Acetobacter aceti strain 1023 and other acetic acid bacteria use succinyl-CoA:acetate CoA-transferase (AarC) in a variant citric acid cycle that is required for a robust acetic acid resistance (aar) phenotype. Strong selection for key roles in acetic acid resistance and central metabolism appear to have optimized the structural and functional properties of AarC, making it an excellent representative of the class I CoA-transferase superfamily. Class I acyl-CoA:carboxylate CoA-transferases produce reactive acylglutamyl anhydride intermediates that acylate CoA, forming either an acyl-CoA product and a free enzyme or a protein glutamyl-CoA thioester and a carboxylate product. A closed active site enables AarC to engage, immobilize, and desolvate acyl-CoA substrates and to stabilize covalent adducts of Glu294.

AarC-N347A lacks the carboxamide moiety proposed to contact the internal oxyanion formed during thiolysis of the acylglutamyl anhydride intermediate. The mutant retains appreciable (~15% of wild-type) specific activity. A data set obtained from a crystal grown in the presence of CoA was used to determine a structure in an orthorhombic space group. All three regions in subunit B adopted the closed conformation. Since AarC-N347A retains significant activity, our hypothesis was that a polar group would simply supplant the missing Asn347 carboxamide and restore its function. As anticipated, an active site solvent molecule was observed at this location in each subunit, with a lower B-factor in subunit B (HOH 775A and 787B: 58 and 34 Å2, respectively). The solvent substitution, however, additionally appears to influence the conformation of Glu294. While Glu294 in the N347A mutant adopts the tt-0 rotamer observed in other closed structures, its χ3 value is unusual, corresponding to a rotation of the attacking oxygen toward the mutated residue (i.e., away from the CoA binding site) [Any value of χ3 is permitted in the Glu tt-0 rotamer]. The resulting misalignment of the key carboxylate may decrease the likelihood of productive nucleophilic attack on an acyl-CoA substrate and affect the reactivity of covalent glutamyl adducts. Without Asn347, Glu294 moves from a position suitable for nucleophilic attack on an acyl-CoA substrate by a carboxylate oxygen syn lone pair to one better aligned for attack by a less-basic and less-nucleophilic anti lone pair.

>MTERIRNVALRSKVCPAETASELIKHGDVVGTSGFTGAGYPKEVPKALAQRMEAAHDRGEKYQISLITGASTGPQLDGELAKANGVYFRSPFNTDATMRNRINAGETEYFDNHLGQVAGRAVQGNYGKFNIALVEATAITEDGGIVPTSSVGNSQTFLNLAEKVIIEVNEWQNPMLEGIHDIWDGNVSGVPTRDIVPIVRADQRVGGPVLRVNPDKIAAIVRTNDRDRNAPFAAPDETAKAIAGYLLDFFGHEVKQNRLPPSLLPLQSGVGNVANAVLEGLKEGPFENLVGYSEVIQDGMLAMLDSGRMRIASASSFSLSPEAAEEINNRMDFFRSKIILRQQDVSASPGIIRRLGCIAMNGMIEADIYGNVNSTRVMGSKMMNGIGGSGDFARSSYLSIFLSPSTAKGGKISAIVPMAAHVDHIMQDAQIFVTEQGLADLRGLSPVQRAREIISKCAHPDYRPMLQDYFDRALKNSFGKHTPHLLTEALSWHQRFIDTGTMLPSSLEHHHHHH[2x]> MDGGMWLMQQINGQVARMKSLGMQLEAADIYNPNGSSLKDAVVMFDGGCTGVLVSNQGLLLTNHHCGYDQIQKHSSVQHNYLKDGFWSYSLAEELVNPGLEVEIVDEITDVTAAVKKELERIKKPSGLEFLSPRYLSSLAPEIVGKKAASRPGYRYEIKAFYGGNRYYMFTKKVFRDVRLVAAPPSSIGKFGSDTDNWAWPRHTGDFSIFRLYADKNGNPAEYSKDNVPYRPKRWVKVNAQGVKEGDFALIMGYPGTTYKFFTADEVTEWSEIDNNIRIEMRGILQDVMLREMLADPKINIMYAAKYASSQNGYKRAQGANWAIRRRSLREIKLAQQQEVLAWAKQKGIATTEEAVRAISKAIEGRQDLRMRQRYLLEGILMGIEMSNAPAADSDIADHWDDPARREAGLQSIRKQFEAFFNKDYSPEVEKDQLAIALLTRYAERIPAEKQPISIREGIAEYGSAKAYVEMIFDKSIYASRERFEEFMKNPDRDRLLRDPMSRFAASVAYEHQKLAKEVAAFDAPLAAAQRSYVASVLDMKGQPNLAPDANLTLRFTYGEIKGYQPRDVVTYGAKSTLEGVMEKEDPNNWEYVVDPKLKALYEAKNYGRYANSDGSMPVNFCATTHTTGGNAGSPVMNARGELIGLNFDRNWEGVGGDIEYLPNYQRSIILDIRYLLFIIDKFAGCQRLIDEIQPQFHHHHHH;> LDV

Here, we show that dipeptidyl peptidase 11 (DPP11), a central metabolic enzyme in these bacteria, undergoes a conformational change upon peptide binding to distinguish substrates from end products. As previously reported, the overall fold of DPP11 comprises a bilobal architecture. The upper helical domain dictates the specificity of the enzyme and caps the catalytic domain, which has a typical chymotrypsin double β-barrel fold. The active site of DPP11 lays in a wide cleft running through the middle of the protein between the catalytic and helical domains, which contributes to the formation of the substrate binding subsites.

We determined the structures for the inactive constructs PgDPP1122-720 S655A, PeDPP1122-717 S652A and its complexes with the dipeptides Arg-Asp and Arg-Glu, as well as the substrate Leu-Asp-Val-Trp, at 2.4, 2.85, 2.2, 2.1 and 2.6 Å resolution, referred to as PgDPP11, PeDPP11, PeDPP11:RD, PeDPP11:RE and PeDPP11:LDVWs, respectively. In PeDPP11:LDVW, the third and fourth amino acids of the substrate (Val and Trp at positions P1′ and P2′, respectively) exhibit few interactions with the enzyme. For instance, Val (P1′) displays a weakly defined electron density with only 40% of its solvent accessible area buried by DPP11, while Trp (P2′) completely lacks electron density. This active site design renders the enzyme’s specificity more relaxed, with selectivity imposed mainly at P1 and P2 residues of the substrate. However, our crystal structures of DPP11 in complex with LDVW and dipeptide RD are both in closed conformation, excluding the possibility that solvent released from the protein’s cleft would explain the larger increase in entropy upon substrate binding. When compared to unbound PeDPP11, the r.m.s.d. of the helical domain is 5-fold higher than that of the catalytic domain for PeDPP11:LDVW and 2-fold higher for PeDPP11:RD and PeDPP11:RE. Particularly, the unfolding of helix α14 (residues 320–346) and loop F441-K451 upon LDVW binding corroborates our hypothesis that protein conformational change is the determining factor for the opposed thermodynamics signatures observed upon peptide binding. Consistent with the measured endothermic binding, we propose that energy is absorbed from the solution to break key interactions, such as those stabilizing loop F441-K451 and intra-main chain polar interactions that stabilize helix α14, but possibly in additional regions of the helical domain. Upon DPP11-substrate binding, the increase in protein conformational entropy counterbalances the overall entropic costs in protein-peptide interactions (including loss of protein and peptide degrees of freedom).> VRVSIERLWSQYFEARAKLGSLEPDEREAAETLEKRVRGLKDRLVVNYSPLVK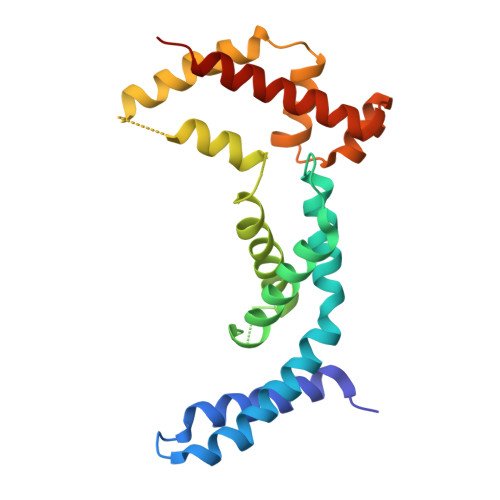YAAGRVTARSTGAVDQEEILSWGILGLLDAVETFDAGKGAKFETYAISKIKWAILDELRRLDXXXXXXXXXXXEAAEIEELRRNLVEAIKNLAERERLVTTFYFYEGLTLREIGKALGLTEGRISQILRQSLGKLRDSLSEPRTS> GPLGSMVATVKRTIRIKTQQHILPEVPPVENFPVRQWSIEIVLLDDEGKEIPATIFDKVIYHLHPTFANPNRTFTDPPFRIEEQGWGGFPLDISVFLL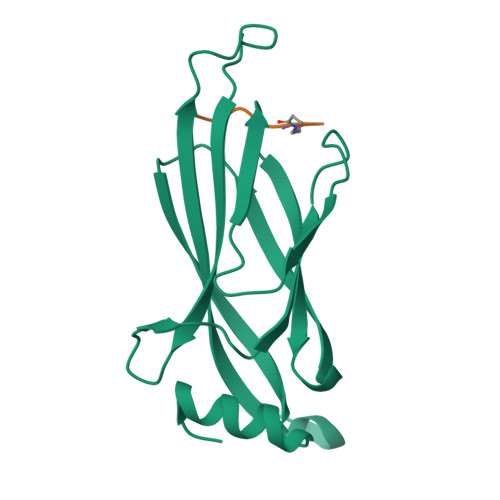EKAGERKIPHDLNFLQESYEVEHVIQIPLNKPLLTEELAKSGST KB2115 | C18 H17 Br2 N O5 | 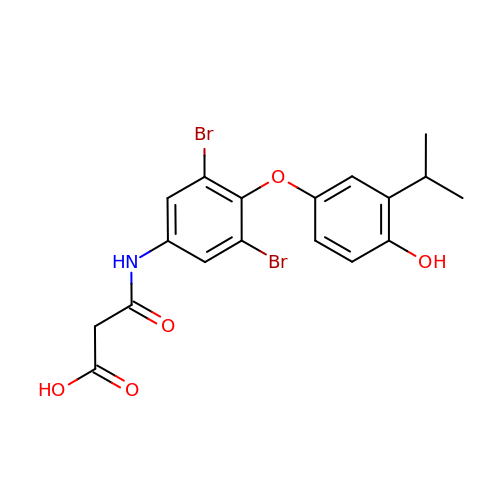VPCSYAVXDAUHLT-UHFFFAOYSA-N> NAVANICQATNSQLYQLVEWAKHIPHFSSLPIEDQVLLLRAGWNELLIAAFSHRSVEVRDGIVLGAGITVHRNSAHQAGVGTIFDRVLTELVAKMRDMNMDRTELGSLRSIILFNPEVRGLKSGQEVELLREKVYAALEEYTRVTR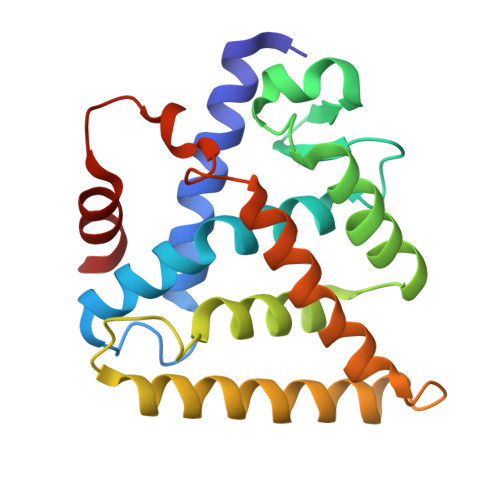PEEPGRFAKLLLRLPALRSIGLKCLEHLFFFKLIGDIPIDTFLMDMLGS>MATCADGRTTANAACCVLFPILDDIQENLFDGAQCGEEVHESLRLTFHDAIGFSPTLGGGGADGSIITFDTIETNFPANAGIDEIVSAQKPFVAKHNISAGDFIQFAGAVGVSNCPGGVRIPFFLGRPDAVAASPDHLVPEPFDSVDTILARMGDAGFSAVEVVWLLASHSIAAADKVDPSIPGTPFDSTPGVFDSQFFIETQLKGRLFPGTPDNKGEVQSPLQGEIRLQSDHLLARDPQTACEWQSMVNNQPKIQNRFAGTMSKMALLGQDKSKLIDCSDIIPTPPALVGAAHLPAGFSLSDVEQACAETPFPALTADPGPVTSVPPVPGS[2x]

The heterologous expression of the POD genes from the P. ostreatus genome, and subsequent kinetic studies, reveal a peroxidase array consisting of three VPs and six MnPs. The VP1 and MnP4 crystal structures were solved as representative for the two POD families present in the P. ostreatus genome. The overall structure of VP1 and MnP4 showed a heme group dividing the protein into a distal largely helical domain (formed by four main helices and two to three small ones) with one structural calcium ion, and a proximal domain composed by another six helices and a non-ordered region stabilized by a second calcium ion. The site where this takes place is conserved and comprises three acidic residues (E36/E40/D175 in VP1 and E36/E40/D181 in MnP4) located near the heme propionate occupying the most internal position with respect to the main access channel.

As already described for P. eryngii VPL, the main structural feature of the P. ostreatus VP1 crystal structure is the combination of the Mn oxidation site of MnPs and the high redox potential substrate oxidation site of LiPs. In addition to the Mn2+ oxidation site, VPs also present a lignin oxidation site, whose presence was detected using VA and RB5 as substrates. This site in VP1 would consist of W164, connected to the heme group via a long-range electron transfer (LRET). The indolic side chain of W164 in VP1 is largely exposed (center) allowing the collection of electrons from the bulky lignin molecule. In a similar way, the W164S mutation in VP1 resulted in a complete loss of activity on VA and RB5 (used as two simple lignin model compounds). The last change in this region concerns S180 in VP1, which is occupied by K186 in MnP4, thus affecting both the surface shape and charge. The lower lip in VP1 presents a clear negative charge and the shape of a wide reservoir, while in MnP4 it displays a less charged surface with a narrow groove (circles in Figure 5C). However, one of the main characteristics of the VP1 structure, when compared with MnP4, is the broader main heme access channel (whose lower lip has the shape of a wide reservoir), which could be related to the reported existence of a third substrate oxidation site in VP. VP1 is the most stable POD retaining over 80% activity after 10 minutes up to 60°C, followed by MnP4, VP3, MnP1, and VP2 (although the VP2 stability sharply decreased with incubation time). For example, we tried to correlate the POD thermal stability to the proline number and position in β-turns and to the effect of heme-apoenzyme bonds. This approach agreed with the fact that VP1 has 12 β-turn prolines (compared with a POD average of nine) and one more heme-apoenzyme bond (than MnP4) but could not be extended to other thermostable P. ostreatus PODs.>MGFAFKRGISTPDLALITRQLATLVQSGMPLEECLRAVAEQSEKPRIRTMLVAVRAK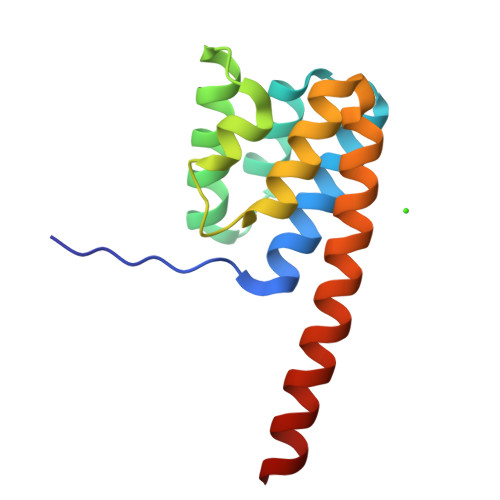VTEGYTLSDSLGDYPHVFDELFRSMVAAGEKSGHLDSVLERLADYAENRQKMRSKLQQASENLYFQ[2x]>MKASDLPLYYNAVDILERNLPVRANKTALFTPDREMTFRQVSNEANQVGNALKGLGVRFGECVGLLTLDSAEWVTSFFGIVKLGAIAVGINTLLKPPEYEYILRDCRARVLIVHQEFLPLIESIRGNLPMLEHIVVIGEGPQEGYLSFNDWIRPQPTTLEAAQSHREDICSLNYSSGTTGGPKGIPHAHKDYPLTAQLWGVNVLGLRESDRTFALAKLFFTFGTGGNLIFPWYVGASCVLFPGAARVASNVLSTISRFKPTIFYNAPTGYAAALALKDFSQHDLSSLRLCVSASEALPAALWYAWKEATGVDIIDGIGCTENFHIFISNRPGDIRPGSSGKPVEGYELKLVDDEGKTVPAGEIGNVLLRSETAALSYWHNFEKSRQTFQGEWLATGDKY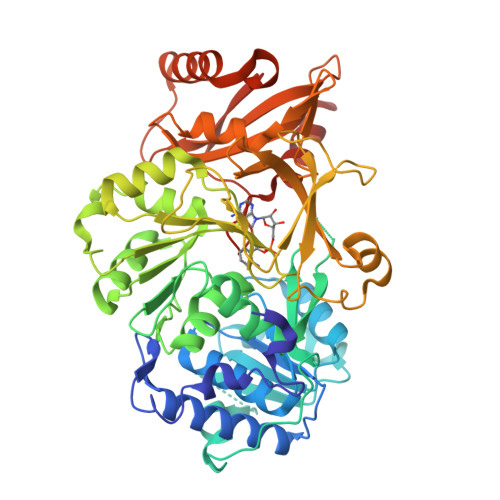FVDADGYYWHAGRSDDMLKVGGIWVSPVEVESTLIQHPAVQECAVIGCPDQSRLIKPKAFIILKPEQIPSEALIRQITDHCTEKMAAYKRPRWIEFVTELPKTATGKIQRFKLRSAAKLAAALEHHHHHH[2x]>GPHMVIRAEKMEAVTHLAASISHEIRNPLTAARGFIQLIEEQPLAADKRRQYARIAIEELDRAEAIITDYLTFAKPAPETPEKLNVKLEIERVIDILRPLANMSCVDIQATLAPFSVIGEREKFRQCLLNVMKNAIEAMPNGGTLQVYVSIDNGRVLIRIADTGVGMTKEQLERLGEPYFTTKGVKGTGLGMMVVYRIIESMNGTIRIESEIHKGTTVSIYLPLASSPSSSTISDKEKQLFAAL[2x];> MKHLSDELLIESYFKAKELNLSPEFIELIEKEIQRRS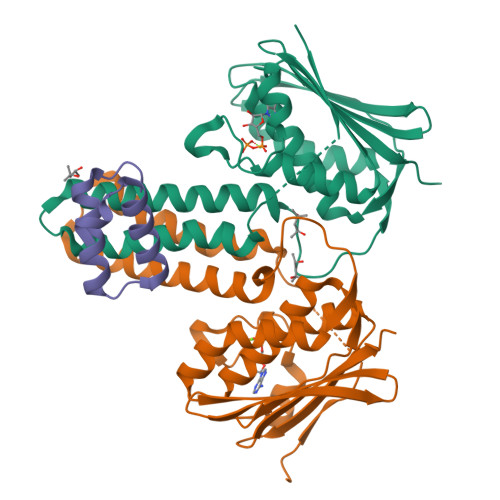LTHKIKLSS>[3x]MSISYRKLDIALSADKETVLVFGQELSTKYFTEIVVTTMLNSTGSDMANSNRILNDIHAAGLDAGDYGKYSRWWAQSNAQERQEAER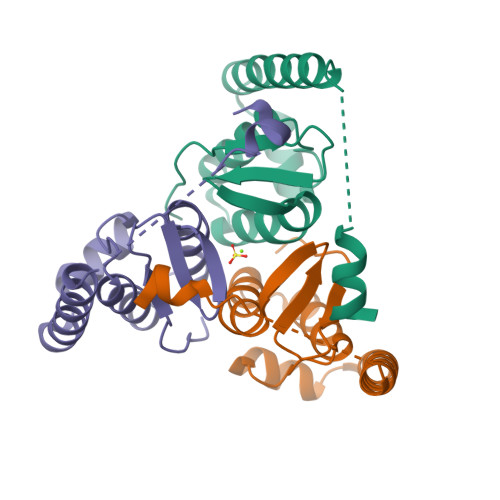RRKEAKAHQERMAAIHATPEEIAKAVAERKAREEALIKRFGNKGAAFGL>[2x]MSEYRPSRPSNPRDDWKLWLVVNPG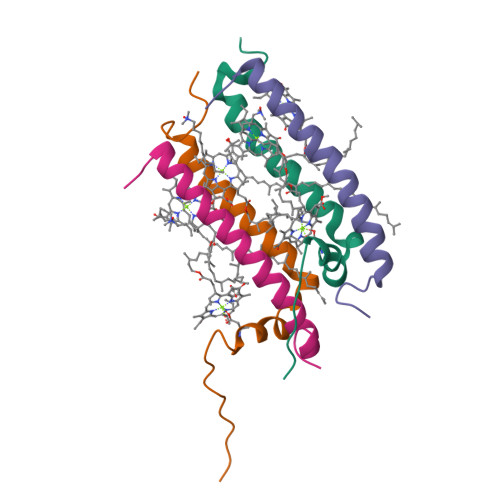TWLIPLLITFLATALIVHSFVFTHEAYNPLTYEVSE;>[2x]MENSISGLTEEQAKEFHEQFKVVFTTFVVLAAAAHFLVFLWRPWF> 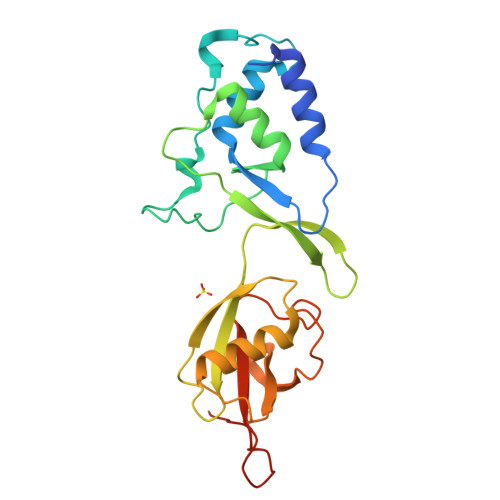MAEGGAADLDTQRSDIATLLKTSLRKGDTWYLVDSRWFKQWKKYVGFDSWDKYQMGDQNVYPGPIDNSGLLKDGDAQSLKEHLIDELDYILLPTEGWNKLVSWYTLMEGQEPIARKVVEQGMFVKHCKVEVYLTELKLCENGNMNNVVTRRFSKADTIDTIEKEIRKIFSIPDEKETRLWNKYMSNTFEPLNKPDSTIQDAGLYQGQVLVIEQKNEDGTWPRLEHHHHHH> GMDTTQVTLIHKILAAADERNLPLWIGGGWAIDARLGRVTRKHDDIDLTFPGERRGELEAIVEMLGGRVMEELDYGFLAEIGDELLDCEPAWWADEAYEIAEAPQGSCPEAAEGVIAGRPV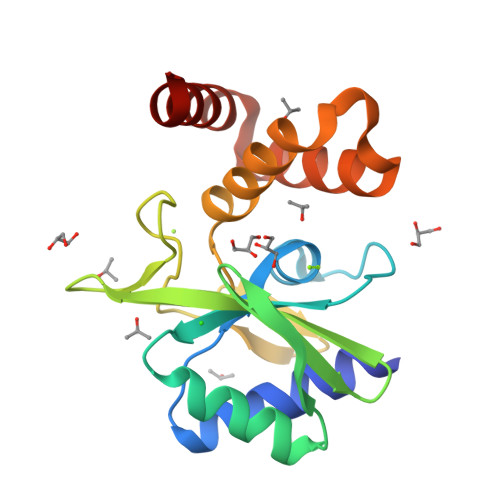RCNSWEAIIWDYFYYADEVPPVDWPTKHIESYRLACTSLGAEKVEVLRAAFRSRYAA>[4x]MGSSHHHHHHSQDPMAIEADSVTRMNELLEILPAKQREILILRVVVGLSAEETAAAVGSTTGAVRVAQHRALQRLKDEIVAAGDYA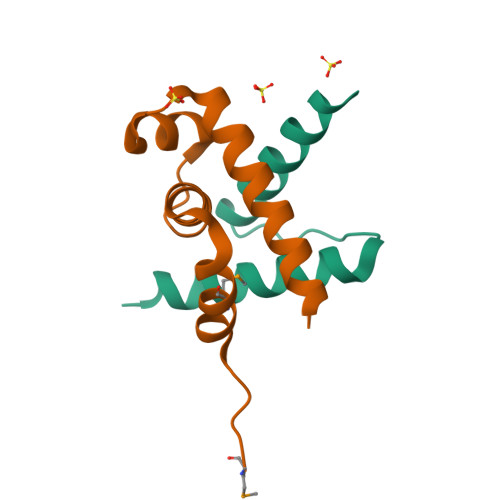;>[4x]MREFGNPLGDRPPLDELARTDLLLDALAEREEVDFADPRDDALAALLGQWRDDLRWPPASALVSQDEAVAALRAGVAQRR>PVMHPHGAPPNHRPWQMKDLQAIKQEVSQAAPGSPQFMQTIRLAVQQFDPTAKDLQDLLQYLCSSLVASLHHQQLDSLISEAETRGITGYNPLAGPLRVQANNPQQQGLRREYQQLWLAAFAALP[3x]

The retroviral structural protein Gag forms the immature protein shell of nascent virus particles4. All retroviral Gag proteins contain three canonical domains: matrix (MA), capsid (CA), consisting of independently folded N-terminal (CA-NTD) and C-terminal (CA-CTD) domains, and nucleocapsid (NC). During immature virus particle formation, these domains function in membrane binding, viral lattice self-assembly and viral genomic RNA (vgRNA) packaging, respectively. Our results show that HTLV-1 uses a distinct CA-NTD arrangement to form the immature Gag lattice and that, in contrast to other retroviral structures, the CA-NTD is the key determinant of immature HTLV-1 assembly.

To analyze the structure of immature HTLV-1 lattice interfaces in more detail, we engineered an HTLV-1 Gag truncation construct for bacterial expression, purification, in vitro assembly and analysis by cryo-ET. The MA126CANC tubes exhibited varying helical parameters. Tubes were sorted into nine groups and each group was processed separately by subtomogram averaging. The in vitro assembled tubes had the same arrangement of the CA-NTD layer as the full-length HTLV-1 Gag VLPs (Cα root-mean-square deviation (r.m.s.d.) = 1.2 Å), underscoring the biological relevance of our in vitro system. The CA-CTD layer in the tubular arrays was arranged in a similar way as in the VLPs produced from cells, also forming a layer of disconnected dimers. However, in this case, the qualitative difference between CA-NTD and CA-CTD was even more dramatic. The CA-CTD density in different individual tubes did not permit structural analysis other than coarse positioning of the CA-CTD dimer, as the CA-CTD layer was only visible at lower resolution (compare Fig. 2d and Extended Data Fig. 6d). Nevertheless, this allowed us to assess large-scale changes in the CA layer between the different tube geometries. Unlike the CA-NTD layer, the CA-CTD layer was observed to have larger movement of its domains. While the distance between the adjacent symmetry-independent CA-NTD trimers was nearly constant (42.1–42.6 Å), the distance between symmetry-independent CA-CTD dimers was skewed such that it was decreased in the direction of tube curvature (31.8 Å) and increased along the tube axis (35.6 Å).Here, we present a high-resolution application of SPA to electron crystallography data, using cryo-EM movies of the prokaryotic, cyclic-nucleotide modulated potassium channel MloK1. Each of the four MloK1 monomers forming the pore has a transmembrane domain (TMD), a voltage sensor domain (VSD), and a soluble cyclic-nucleotide binding domain (CNBD), which lies in the intracellular side. The total molecular weight of the tetramer is 160 kDa. Furthermore, we identified different conformations of MloK1 tetramers within the disordered 2D crystals by means of single-particle classification.

Although the 2D crystal images processed did not diffract beyond 10 Å, we improved the resolution of the MloK1 3D map to 4.0 Å. The overall resolution of the map improved from 4.5 to 4.0 Å using our single-particle approach. The map's resolution is better in the xy membrane plane than it is along the z axis. The refined map contains nine full MloK1 tetramers. Even though the missing cone effect is still present, and images of tilted samples are generally of lower quality than of non-tilted samples, the application of SPA algorithms to the MloK1 dataset ameliorated the overall resolution by accounting for local variations in the tilt geometries along the distorted 2D crystals, thus offering a higher diversity of views for the 3D reconstruction. Our highest resolution structure, derived from the consensus map, is in general agreement with our previously published model. However, we here show that the previously determined structure was an average of several coexisting conformations. The procedure allows retrieving high-resolution information from disordered and non-flat 2D crystals, as illustrated by the 4 Å consensus model presented.

>[4x]MSVLPFLRIYAPLNAVLAAPGLLAVAALTIPDMSGRSRLALAALLAVIWGAYLLQLAATLLKRRAGVVRDRTPKIAIDVLAVLVPLAAFLLDGSPDWSLYCAVWLLKPLRDSTFFPVLGRVLANEARNLIGVTTLFGVVLFAVALAAYVIERDIQPEKFGSIPQAMWWAVVTLSTTGYGDTIPQSFAGRVLAGAVMMSGIGIFGLWAGILATGFYQEVRRGDFVRNWQLVAAVPLFQKLGPAVLVEIVRALRARTVPAGAVICRIGEPGDRMFFVVEGSVSVATPNPVELGPGAFFGEMALISGEPRSATVSAATTVSLLSLHSADFQMLCSSSPEIAEIFRKTALERRGAAASA> SGYTEDEKLNIAKRHLLPKQIERNALKKGELTVDDSAIIGIIRYYTREAGVRGLEREISKLCRKA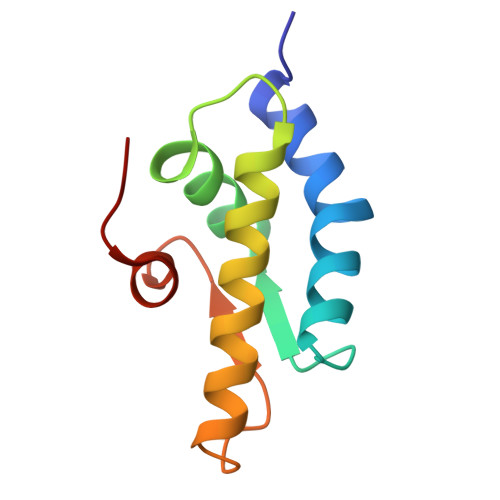VKQLLLDKSLKHIEINGDNLHDYLGVQRF> MELKHSISDYTEAEFLQLVTTICNADTSSEEELVKLVTHFEEMTEHPSGSDLIYYPKEGDDDSPSGIVNTVKQWRAANGKSGFKQGLEHHHHH;> MESKRNKPGKATGKGKPVGDKWLDDAGKDSGAPIPDRIADKLRDKEFKSFDDFRKAVWE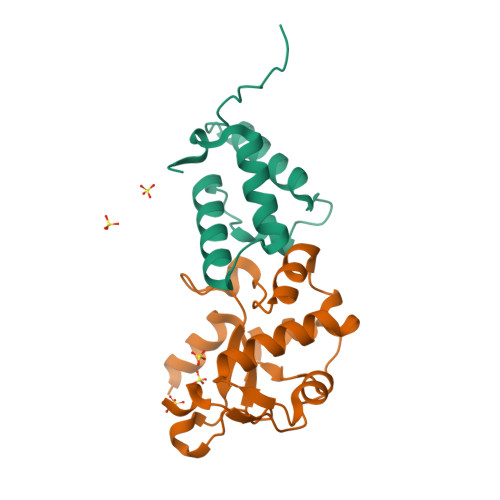EVSKDPELSKNLNPSNKSSVSKGYSPFTPKNQQVGGRAVYELHHDKPISQGGEVYDMDNIRVTTPKRHIDIHRGK> SMFGCLVAGRLVQTAAQQVAEDKF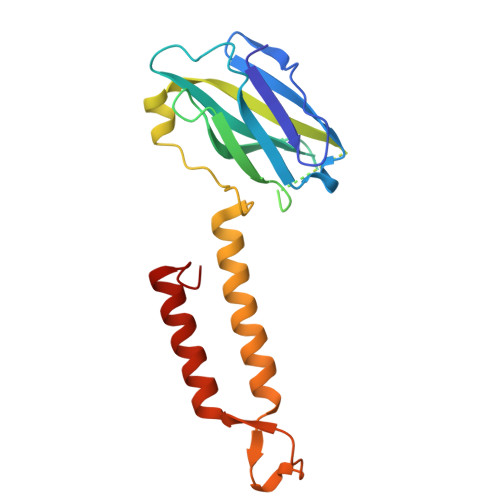VFDLPDYESINHVVVFMLGTIPFPEGMGGSVYFSYPDSNGMPVWQLLGFVTNGKPSAIFKISGLKSGEGSQHPAGAMNIVRTPSVAQIGISVELLDSMAQQTPVGNAAVSSVDSFTQFTQKMLDNFYNFASSFAVSQAQMTPSPSEMFIPANVVLKWYENFQRRLAQNPLFWKT>MGSSHHHHHHMEELDRSRAFARDVKRIVVKVGTAVVTGKGGRLALGRLGALCEQLAELNSDGFEVILVSSGAVGLGRQRLRYRQLVNSSFADLQKPQTELDGKACAGVGQSSLMAYYETMFDQLDVTAAQLLVNDSSFRDKDFRKQLNETVKSMLDLRVIPIFNENDAISTRRAPYQDSSGIFWDNDSLAALLALELKADLLILLSDVEGLYTGPPSDPNSKLIHTFVKEKHQDEITFGDKSRLGRGGMTAKVKAAVNAAYAGIPVIITSGYSAENIDKVLRGLRVGTLFHQDARLWAPITDSNARDMAVAARESSRKLQALSSEDRKKILLDIADALEANVTTIKAENELDVASAQEAGLEESMVARLVMTPGKISSLAASVRKLADMEDPIGRVLKKTEVADGLVLEKTSSPLGVLLIVFESRPDALVQIASLAIRSGNGLLLKGGKEARRSNAILHKVITDAIPETVGGKLIGLVTSREEIPDLLKLDDVIDLVIPRGSNKLVTQIKNTTKIPVLGHADGICHVYVDKACDTDMAKRIVSDAKLDYPAACNAMETLLVHKDLEQNAVLNELIFALQSNGVTLYGGPRASKILNIPEARSFNHEYCAKACTVEVVEDVYGAIDHIHRHGSAHTDCIVTEDHEVAELFLRQVDSAAVFHNASTRFSDGFRFGLGAEVGVSTGRIHARGPVGVEGLLTTRWIMRGKGQVVDGDNGIVYTHQDIPIQA[8x]

Delta-1-pyrroline-5-carboxylate synthase (P5CS) is a key enzyme in proline biosynthesis pathway. This enzyme catalyses a two-step reaction that converts glutamate to l-glutamate-5-phosphate (G5P) and then to l-glutamate-5-semialdehyde. l-Glutamate-5-semialdehyde will spontaneously cyclize and reach equilibrium with delta-1-pyrroline-5-carboxylate (P5C). As a bifunctional enzyme, P5CS has two structural domains: the glutamate kinase (GK) domain and the glutamyl phosphate reductase (GPR) domain. Our results show that Arabidopsis thaliana P5CS1 (AtP5CS1) and P5CS2 (AtP5CS2) can form enzymatic filaments in a substrate-sensitive manner.

After obtaining active protein, we prepared cryo-samples of mixed-state AtP5CS1. Similar to the AtP5CS2 filament, the AtP5CS1 filament is composed of tetramers serving as the basic helical unit. Adjacent helical units interact through assembly interfaces comprising hooks. Differing from the AtP5CS2 filament, the adjacent helical units in the AtP5CS1 filament do not assemble in a completely perpendicular manner. The helical twist is slightly smaller, approximately 80°. In the resolved density map of AtP5CS1, stable density for the GK region was obtained. According to our model, the GPR domain of AtP5CS1 is positioned closer to GK. In the model of AtP5CS1, the substrate ATP has been captured. Similar to the ADP binding in AtP5CS2, the adenine group is stabilized by the ATP binding loop of AtP5CS1, and the triphosphate group interacts with the conserved functional amino acids K20, D177 and K242. We identified a small density located near the RGP binding amino acids S60, A62 and D157, implying that this could be the density of the substrate glutamate.>[2x]MAGAIKVGTWGGNGGSEWD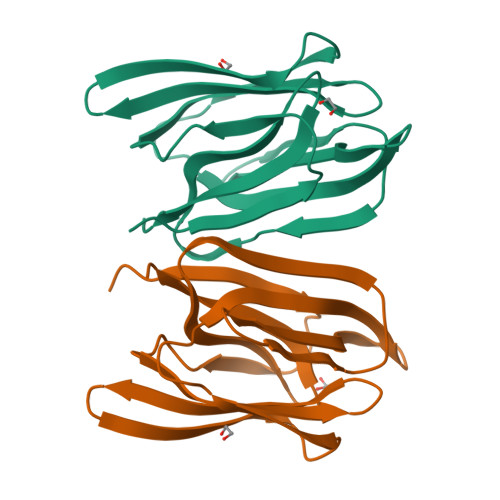MGPAYRIDSVKINAGDIIDAIEITFTRYGLTETQHYGGTGGEPHEIAFEDGEYIMSMEGHVVDYFGLTIIGKLTLTTNRRTFGPFGAYEGTPFSIPVAEGKIAGFFGRAGSFIDAIGVYLMPNLEHHHHHH>DIKKILPHRYPFLLVDKVIYMQPNKTIIGLKQVSTNEPFFNGHFPQKQIMPGVLQIEALAQLAG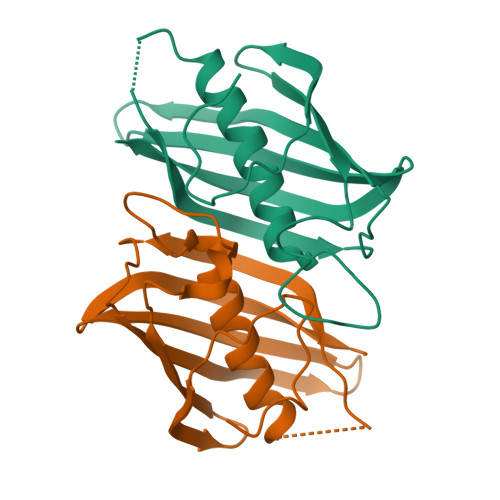ILCLKSDDSQKNNLFLFAGVDGVRWKKPVLPGDTLTMQANLISFKSSLGIAKLSGVGYVNGKVVINISEMTFALS[2x]3,3'-[(3-carboxy-4-oxocyclohexa-2,5-dien-1-ylidene)methylene]bis(6-hydroxybenzoic 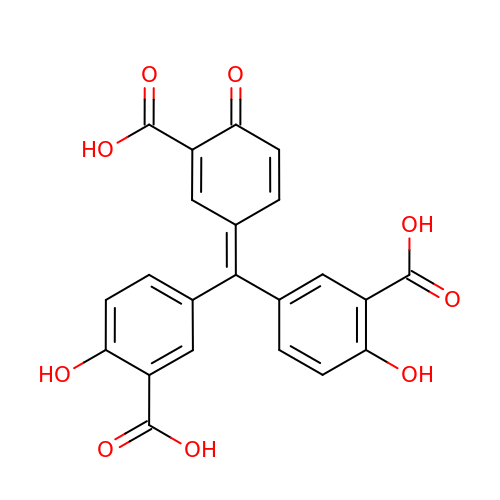acid) | C22 H14 O9 | GIXWDMTZECRIJT-UHFFFAOYSA-N As antigen receptors, the lamprey utilize a family of highly diverse proteins called variable lymphocyte receptors (VLRs), which contain multiple, tandem leucine-rich repeat (LRR) motifs. The resulting VLRB protein is a 15–25 kDa, crescent-shaped protein with a continuous beta sheet where its concave surface forms the antigen binding site. Herein, we report on the characterization of a lamprey VLRB that is specific for terminal 3-O-SGal, and was isolated from a lamprey immunized with human type O erythrocytes. This VLRB, termed O6, is the first reagent to our knowledge that specifically recognizes the 3-O-SGal determinant on glycoproteins with high sensitivity. To better understand the molecular determinants of glycan recognition, we determined crystal structures of unliganded (apo) O6 and a co-crystal structure of O6 in complex with (3 S)Galβ1-4GlcNAc. This O6 VLR is relatively small compared to other characterized VLRBs, containing 178 amino acids (~19.2 kDa) and only a single LRR variable domain (LRRV1) along with the other usual LRR and CP components (LRRNT, LRR1, LRRVe, CP, and LRRCT).

The structure of O6 in complex with (3 S)Galβ1-4GlcNAc at 1.9 Å resolution provides a detailed view of sulfated glycan recognition by this VLR. The sulfate group of the ligand forms hydrogen bonds with Gln86, His109, and the backbone amide of Gly137 in an identical manner to a phosphate ion in the apo structure. Specifically, Asp85 and Ser61 hydrogen bond to the 4-OH and 6-OH of Gal, respectively. The side-chain NH of Trp35 hydrogen bonds with 3-OH of GlcNAc, while Asp16 hydrogen bonds with the nitrogen of the GlcNAc acetamide group. Two water molecules mediate interactions between Ser37 and Asn62 and GlcNAc and Gal hydroxyl and O groups. Trp138 of the C-terminal loop packs against the face of the GlcNAc residue, a feature that has been observed in all glycan-binding VLRs to date. The binding interactions observed in the crystal structure are consistent with the CFG glycan array and ITC data where VLR O6 makes specific interactions with 3-OH of GlcNAc and the 3-SO3, 4-OH, and 6-OH of Gal. The 2-OH of Gal, 6-OH and 1-OH of GlcNAc remain open for substitution or glycosidic linkage. Comparison of the apo and glycan complexes shows no movement of the C-terminal loop and only small changes in residue rotamers (including Trp138), indicating that the VLR is preconfigured for glycan binding (RMSD 0.28 Å for 172 aligned residues).

>[2x]GSCPSQCSCSGTDVNCDGARFASVPAAIPITTQRLWLSNNQLTKLDPGVFDSLTQLTTLYLSNNQLTALPAGVFDKLTQLKELGLDQNQLKSIPDGAFARLPSLTHVWLHTNPWDCQCTDILYLSGWVAQHSSIVGEGWLRSWTVNPDNAKCSGTNTPVRAVTEASTSPSKCP> SAKELRCQCIKTYSKPFHPKFIKELRVIESGPHCANTE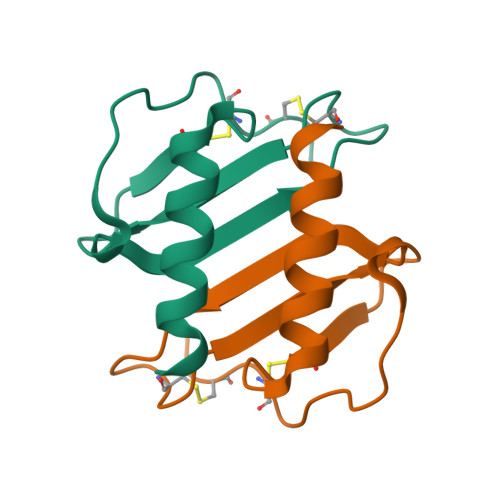IIVKLSDGRELCLDPKENWVQRVVEKFLKRAENS Members of the family Birnaviridae possess bi-segmented double-stranded RNA (dsRNA) genomes and form virions with non-enveloped single-shelled icosahedral capsids. From sequence analysis it was proposed that the RdRPs of Birnaviridae possess a non-canonical active site where the polymerase sequence motifs are re-ordered C-A-B, motif C containing ADN in place of the conserved GDD catalytic residues. An additional unusual feature of birnavirus RdRPs is their ability to self-guanylylate: auto-catalyzing the covalent addition of a GMP moiety to a serine residue of the polymerase in a template-independent manner to form VP1pG. We have cloned, expressed and solved the structure of the RdRP VP1 from IPNV in both its apo form and bound to a catalytic metal (magnesium).

We have expressed and purified the IPNV RNA-dependent RNA polymerase VP1 and determined its structure to 2.2 Å resolution. To characterize binding of catalytic metals at the active site of the enzyme, crystals of ΔC55 VP1 were soaked in reservoir solution supplemented with 50 mM MgCl2 and 10 µM GTP and lacking citrate (which chelated metals, frustrating soaking experiments). A single Mg2+ ion was observed bound at the active site, coordinated by four solvent molecules and the side chain oxygen atoms of N389 and D402 in an octahedral geometry. The coordination geometry of the bound K+ ion does not change upon addition of Mg2+, suggesting that Mg2+ does not replace K+ in this position. As in the structure of IBDV VP1 soaked with Mg2+ and GTP, no significant structural rearrangements were observed between the structures of apo and Mg-bound ΔC55 VP1 and no electron density for a bound GTP molecule was observed. However, when soaked with an excess of Mg2+ ions we observe only one Mg2+ ion at the active site, coordinated by the side chains of N389 and D402. We performed additional experiments, soaking ΔC55 IPNV VP1 crystals with up to 200 mM Mg2+ and 40 mM Mn2+, but these failed to reveal any additional bound Mg2+ (data not shown). In the structure of reovirus RdRP solved in the absence of substrate nucleotides a single Mn2+ ion is observed in the active site in a position corresponding to that we observe for the single Mg2+ of IPNV VP1, being coordinated by the side chains of D735, D585 and E780 (equivalent to VP1 residues N389, D402 and half-way between D559 and S400, respectively). Upon formation of an initiation complex two Mn2+ ions bind the reovirus RdRP active site. It is therefore likely that in the presence of template and nucleotide substrates a second metal ion will bind at the active site of IPNV VP1 and the resulting initiation complex will contain two metal ions coordinated by D388, D402 and the nucleotide triphosphate moiety at the tip of the catalytic motif C β hairpin.

>MSDIFNSPQNKASILTALMKSTTGDVEDVLIPKRFRPAKDPLDSPQAAAQFLKDNKYRILRPRAIPTMVELETDAALPRLRQMVEDGKLKDTVSVPEGTTAFYPKYYPFHKPDHDEVGTFGAPDITLLKQLTFFLLENDFPTGPETLRQVREAIATLQYGSGSYSGQLNRLLAMKGVATGRNPNKTPKTVGYTNEQLAKLLEQTLPINTPKHEDPDLRWAPSWLINYTGDLSTDKSYLPHVTIKSSAGLPYIGKTKGDTTAEALVLADSFIRDLGRAATSADPEAGVKKTITDFWYLSCGLLFPKGERYTQVDWDKKTRNIWSAPYPTHLLLSMVSTPVMNESKLNITNTQTPSLYGFSPFHGGMDRIMTIIRDSLDNDEDLVMIYADNIYILQDNTWYSIDLEKGEANCTPQHMQAMMYYLLTRGWTNEDGSPRYNPTWATFAMNVAPSMVVDSSCLLMNLQLKTYGQGSGNAFTFLNNHLMSTIVVAEWVKAGKPNPMTKEFMDLEEKTGINFKIERELKNLRETIVEAVETAPQDGYLADGSDLPPIRPGKAVELDLLGWSAIYSRQMEMFVPVLENERLIASAAYPKGLENKALARKPGAEIAYQIVRYEAIRLVGGWNNPLLETAAKHMSLDKRKRLEVKGIDVTGFLDDWNNMSEFGGDLEGITLSEPLTNQTLVDINTPLDSFDPKARPQTPRSPKKTLDEVTTAITSGTYKDPKSAVWRLLDQRTKLRVSTLRDQALALKPASSSVDNWAEATEELAQQQQLLMKANNLLKSSLTETREALEKTGHHHHHH[5x]To date, more than 10 MARTX effector domains have been annotated, including several domains of unknown function in Vibrio species, among which the fifth domain of a MARTX toxin from Vibrio vulnificus CMCP6 is a Ras/Rap1-specific endopeptidase (RRSP). RRSP catalyzes sequence-specific cleavage of the Switch I region of the cellular substrates Ras and Rap1 (18, 19) that are critical for a myriad of signal transduction events, including innate immune defenses. Structural and functional bioinformatics and cell biological studies revealed that RRSP belongs to the TIKI superfamily, and it is composed of an N-terminal region mediating its localization to the plasma membrane and a C-terminal region responsible for cytotoxicity. In this study, we determined the crystal structure of an RRSP from the sepsis-causing pathogen V. vulnificus CMCP6 (VvRRSP), and we demonstrated that it is a metal-independent TIKI family endopeptidase.

Given that the catalytic residues of VvRRSP were successfully assigned, we hypothesized that substitution of catalytic residues with nonfunctional residues might stabilize the active site and the adjacent flexible region. We subsequently determined the structure of the RRSPE3930L/H4030L mutant at a resolution of 2.3 Å. The structure of the mutant RRSP is essentially identical to that of WT RRSP (RMSD of Cα atoms is less than 0.5 Å), with minimal differences in the conformation of the active sites containing the essential residues. Like WT RRSP, the active site of the VvRRSPE3930L/H4030L mutant is arranged similarly to that of BcR135. Luckily, the flexible region spanning residues Arg-3988–Gln-3992 in molecule A of the mutant is ordered and adopts a loop structure close to the active site. To evaluate the involvement of this region in the function of RRSP, we selected Arg-3988 based on its interactions with the Switch I region of Ras, dominated by negatively charged residues. This residue was mutated to glutamate, and the overall conformation was confirmed by CD spectroscopy. In vitro KRas cleavage assays showed that the mutation completely inhibited enzymatic activity, suggesting that the flexible loop may be involved in substrate recognition. No differences in the active sites were observed between WT and mutant RRSP structures. Therefore, these results suggest that residues Glu-3900, Glu-3930, His-3902, and His-4030 in the active site may spontaneously adopt the catalytically active conformation in the presence of substrate.

>[4x]GAMAQELKERAKVFAKPIGASYQGILDQLDLVHQAKGRDQIAASFELNKKINDYIAEHPTSGRNQALTQLKEQVTSALFIGKMQVAQAGIDAIAQTRPELAARIFMVAIEEANGKHVGLTDMMVRWANEDPYLAPKHGYKGETPSDLGFDAKYHVDLGEHYADFKQWLETSQSNGLLSKATLDESTKTVHLGYSYQELQDLTGAESVQMAFYFLKEAAKKADPISGDSAEMILLKKFADQSYLSQLDSDRMDQIEGIYRSSHETDIDAWDRRYSGTGYDELTNKLASATGVDEQLAVLLDDRKGLLIGEVHGSDVNGLRFVNEQMDALKKQGVTVIGLLHLRSDLAQPLIDRYLATGVMSSELSAMLKTKHLDVTLFENARANGMRIVALDANSSARPNVQGTEHGLMYRAGAANNIAVEVLQNLPDGEKFVAIYGKALLQSHKGIEGFVPGITHRLDLPALKVSDSNQFTVEQDDVSLRV> MRGSHHHHHHTDPAYVPAPGYQPTYNPTLPYKRPIPGGLSVGMSVYIQGMAKEN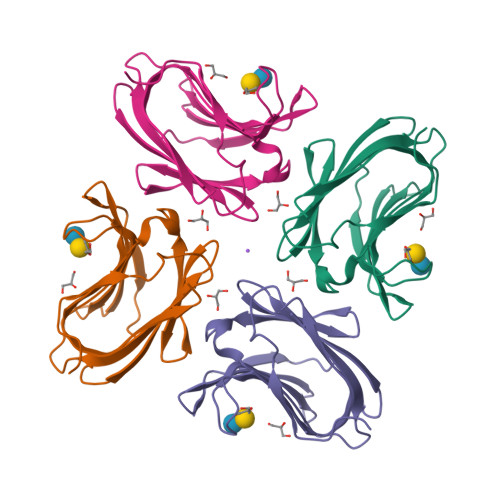MRRFHVNFAVGQDDGADVAFHFNPRFDGWDKVVFNTMQSGQWGKEEKKKSMPFQKGKHFELVFMVMPEHYKVVVNGNSFYEYGHRLPVQMVTHLQVDGDLELQSINFLGG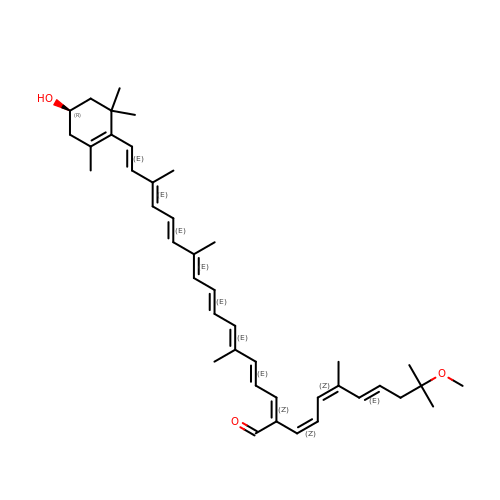(2~{Z},4~{E},6~{E},8~{E},10~{E},12~{E},14~{E},16~{E})-2-[(1~{Z},3~{Z},5~{E})-8-methoxy-4,8-dimethyl-nona-1,3,5-trienyl]-6,11,15-trimethyl-17-[(4~{R})-2,6,6-trimethyl-4-oxidanyl-cyclohexen-1-yl]heptadeca-2,4,6,8,10,12,14,16-octaenal | C41 H56 O3 | DFOYVSCLGRVGJK-PCDZQMFBSA-N> GSHMNNDFNGKITLAITGASGASYAMRLIECLIAANYQLYILCSSAGRISLDTEVG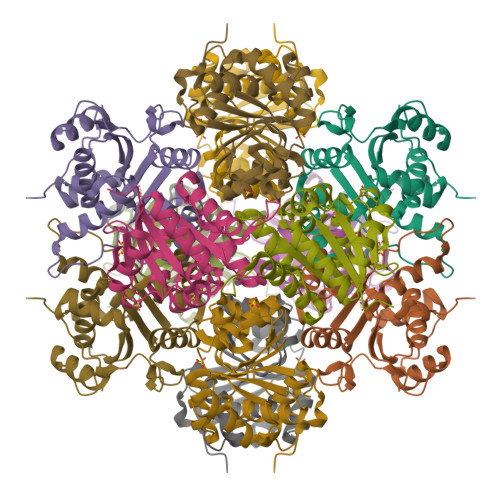VKIPSSPDAASKFLTEKYQAKDQQITVFGKEQWFSPVASGSSAPKQMVVCPCSTGTMAAICHGMSDNLIERAADVVIKERGQLILMVRETPFSTLHLQNMLSLSQQGVTIMPASPGFYHKVETIEDLIDFMVGRVLDHLGIEQDIMPRWGYNI trimethylamine oxide 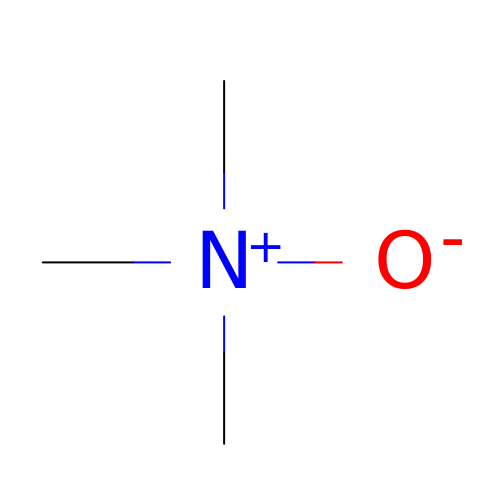| C3 H9 N O | UYPYRKYUKCHHIB-UHFFFAOYSA-N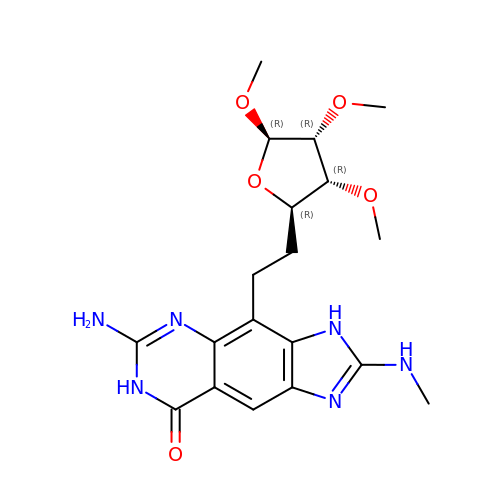6-amino-2-(methylamino)-4-(2-((2R,3R,4R,5R)-3,4,5-trimethoxytetrahydrofuran-2-yl)ethyl)-1H-imidazo[4,5-g]quinazolin-8(7H)-one | C19 H26 N6 O5 | OMBPYCFBGGXDQG-BNGXUDDSSA-N The dimeric two-pore OSCA/TMEM63 family has recently been identified as mechanically activated ion channels. In our previous work, we identified OSCA/TMEM63 as a conserved family of MA ion channels spanning several eukaryotic clades and having considerable diversity in the plant kingdom, where species commonly have more than one paralog. Similar to the TMEM16 family, OSCAs are dimeric and each subunit has a pore lined by transmembrane helices (TMs) 3–7, instead of a single pore along the symmetry axes. A hydrophobic gate on the extracellular half of the pore blocks ion flow.

Here, we used cryo-EM to determine a high-resolution structure of AtOSCA3.1, the first reported OSCA gene, in nanodiscs. Purified protein was then reconstituted into nanodiscs and subjected to cryo-EM analysis, resulting in a 2.6 Å resolution symmetric reconstruction sufficient to build a model of the majority of the protein (537 out of 724 residues) Due to increased flexibility of the BLD relative to previous OSCA structures, we were unable to assign residue identity, and instead modeled it as two poly-Ala helices. Overall, there is good agreement between OSCA3.1, OSCA1.1 and OSCA1.2 protomers (Cα RMSD OSCA3.1-OSCA1.1: 1.243 Å, OSCA3.1-OSCA1.2: 1.152 Å). The pore profile of these OSCAs is maintained and the small radii towards the extracellular side suggests these channels are in a closed/non-conductive state, as suggested by previous MD simulations (Jojoa-Cruz et al., 2018; Zhang et al., 2018). Likewise, the two π-helical turns in TM5 and TM6a seen in previous structures near the neck of the pore are present at similar positions in OSCA3.1. We identified multiple lipid-like densities in one of our postprocessed maps. Notably, one of these densities is located at the pore fenestration, at a position similar to that observed in previous MD simulations of OSCA1.2, supporting the proposed occupation of the pore pathway by lipids. Lipids were tentatively modeled as palmitic acid (green), phosphatidylcholine (cyan), and lyso-phosphatidylethanolamine (purple). However, the inter-subunit cleft in the nanodisc structure is wider due to outward movements of innermost TMs ranging from ~4–8 Å relative to the digitonin sample, which was recently denoted as an ‘extended’ state. Thus, our nanodisc structure represents a further ‘extended’ state than the one found both in digitonin and LMNG micelles (Zhang et al., 2023).

>[2x]MEFGSFLVSLGTSFVIFVILMLLFTWLSRKSGNAPIYYPNRILKGLEPWEGTSLTRNPFAWMREALTSSEQDVVNLSGVDTAVHFVFLSTVLGIFACSSLLLLPTLLPLAATDNNIKNTKNATDTTSKGTFSQLDNLSMANITKKSSRLWAFLGAVYWISLVTYFFLWKAYKHVSSLRAQALMSADVKPEQFAILVRDMPAPPDGQTQKEFIDSYFREIYPETFYRSLVATENXXXXXXXXXXXXXKKKLARAEAILAATNNRPTNKTGFCGLVGKQVDXXXXXXXXXXXXXXXXXXXXXXXXAEKQQTAAVVFFTTRVAAASAAQSLHCQMVDKWTVTEAPEPRQLLWQNLNIKLFSRIIRQYFIYFFVAVTILFYMIPIAFVSAITTLKNLQRIIPFIKPVVEITAIRTVLESFLPQIALIVFLAMLPKLLLFLSKAEGIPSQSHAIRAASGKYFYFSVFNVFIGVTLAGTLFNTVKDIAKNPKLDMIINLLATSLPKSATFFLTYVALKFFIGYGLELSRIIPLIIFHLKKKYLCKTEAEVKEAWYPGDLSYATRVPGDMLILTITFCYSVIAPLILIFGITYFGLGWLVLRNQALKVYVPSYESYGRMWPHIHQRILAALFLFQVVMFGYLGAKTFFYTALVIPLIITSLIFGYVCRQKFYGGFEHTALEVACRELKQSPDLEEIFRAYIPHSLSSHKPEEHEFKGAMSRYQDFNAIAGVGTGTLEVLFQ> MVEQMLSKNMLLGGFDTGNIKAKISFLNEKGNIESFAIPTVIAEAPPAKIDLKSAPSKKNDYVNEKDEDIELLHVRIISNSLDGDARSRAWYVGAYAKDQEDRQEPTVDEMGKTEDKFSQKNKKLHLIPLFTSMAVAAARIGKEEVSVPFSGGMPIEDYKLRGEEQILEMLYGEHTVEFLDGTYEGKKIKITINDGTMNVEG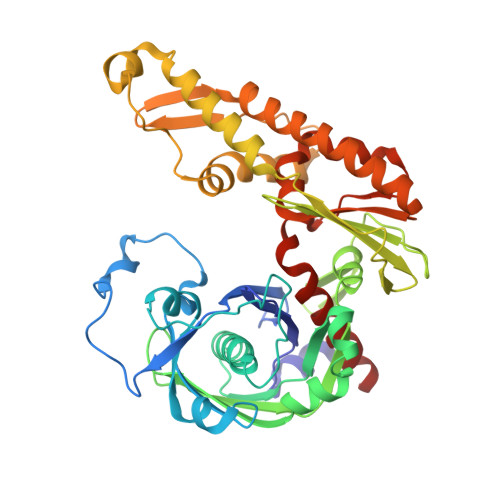VSSVLAILFDIVNGEIVEVEGMDAEIGESYAINDLGAGTSDNAFFEDGELNKKLSTNTDLGTNKYIDEILKNIKERFMENEILKSFMTDEIESPFKTREDFIQRLVMPEVEKMIEDDTYKPTFSVKWGPVKENVTDIVMDGMLKYAEDQKASLMKFWFKTNADKNIVVGGGVLFGYAGLRDLKEQDGFILPKNIQESAYFTSRSYLIANLLEQLNKEGVEA> MAAIDKLVKASHLIDMNDIIREGNPTLRKVAEEVTFPLSEKEEILGEKMMQFLKHSQDPIMAEKLGLRGGVGLAAPQLDISKRIIAVLVPNVEDAQGNPPKEAYSLQEVMYNPKVVSHSVQDAALSDGEGCLSVDREV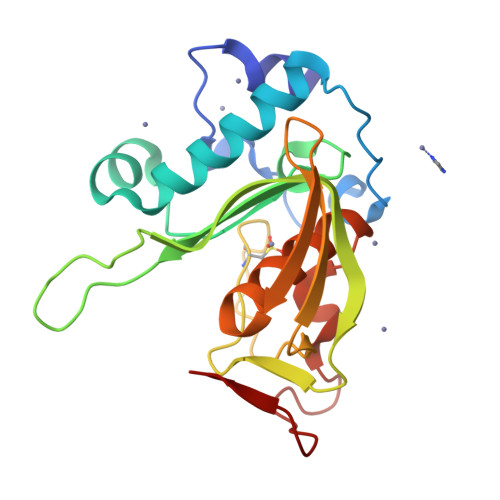PGYVVRHARVTIEYFDKTGEKHRLKLKGYNSIVVQHEIDHIDGIMFYDRINEKNPFAVKEGLLILE Ruminococcus gnavus is a human gut symbiont wherein the ability to degrade mucins is mediated by an intramolecular trans-sialidase (RgNanH). RgNanH comprises a GH33 catalytic domain and a sialic acid-binding carbohydrate-binding module (CBM40). RgCBM40 displays the canonical CBM40 β-sandwich fold and broad specificity towards sialoglycans with millimolar binding affinity towards α2,3- or α2,6-sialyllactose. RgCBM40 binds to mucus produced by goblet cells and to purified mucins, providing direct evidence for a CBM40 as a novel bacterial mucus adhesin.

Protein ligand complexes were achieved for both 3′SL and 6′SL. Definitive electron density for the Neu5Ac and galactose residues was observed in the 3′SL and 6′SL complexes. In the 6′SL complex, electron density was also observed for the glucose residues, with the lactose positioned almost perpendicular to the sialic acid. Due to the glycan orientation introduced by the α2-6-sialic acid linkage the 6′SL glucose residue is close to the protein surface. Therefore, α2-6-linked LacNAc N-acetyl group may be blocked by protein residues, whereas the α2-3 linked glycan would be more solvent exposed. In the 3′SL complex, the lactose positioning would permit further extensions to the carbohydrate chain as would be present in more complex or anchored glycans, whereas these may be blocked in the 6′SL complex. This would provide a degree of specificity towards sialic acid linkage. The affinity of the interaction between RgCBM40 and sialic acid ligands was further assessed by ITC. Both 3′SL and 6′SL bound with similar low affinities, with dissociation constants of 0.57 mM and 1.70 mM, respectively. Furthermore, it would suggest that the additional binding interactions observed in the crystal structure of the complex between RgCBM40 and 6′SL do not significantly promote binding, also in agreement with the STD NMR results, showing that sialic acid is the main binding epitope in solution. In the RgCBM40 complex crystal structures, sialic acid is bound in the α-anomeric conformation, allowing the axial C2 carboxylic acid moiety to form a conserved interaction with Arg204.

>MADIGSVLQKEGIEISEGTGYDLSKEPGAATVKALEQGTIVISYKTTSENAIQSLLSVGNGTKGNQDRHFHLYITNAGGVGMELRNTDGEFKYTLDCPAAVRGSYKGERVSNTVALKADKENKQYKLFANGELIATLDQEAFKFISDITGVDNVMLGGTMRQGTVAYPFGGSIERMQVYRDVLSDDELIAVTGK[2x]>[6x]MGHHHHHHQQLASFLSGTWQSGRGRSRLIHHAISGEALWEVTSEGLDMAAARQFAIEKGAPALRAMTFIERAAMLKAVAKHLLSEKERFYALSAQTGATRADSWVDIEGGIGTLFTYASLGSRELPDDTLWPEDELIPLSKEGGFAARHLLTSKSGVAVHINAFNFPCWGMLEKLAPTWLGGMPAIIKPATATAQLTQAMVKSIVDSGLVPEGAISLICGSAGDLLDHLDSQDVVTFTGSAATGQMLRVQPNIVAKSIPFTMEADSLNCCVLGEDVTPDQPEFALFIREVVREMTTKAGQKCTAIRRIIVPQALVNAVSDALVARLQKVVVGDPAQEGVKMGALVNAEQRADVQEKVNILLAAGCEIRLGGQADLSAAGAFFPPTLLYCPQPDETPAVHATEAFGPVATLMPAQNQRHALQLACAGGGSLAGTLVTADPQIARQFIADAARTHGRIQILNEESAKESTGHGSPLPQLVHGGPGRAGGGEELGGLRAVKHYMQRTAVQGSPTMLAAISKQWVRGAKVEEDRIHPFRKYFEELQPGDSLLTPRRTMTEADIVNFACLSGDHFYAHMDKIAAAESIFGERVVHGYFVLSAAAGLFVDAGVGPVIANYGLESLRFIEPVKPGDTIQVRLTCKRKTLKKQRSAEEKPTGVVEWAVEVFNQHQTPVALYSILTLVARQHGDFVD

PaaZ is a fusion of N-terminal aldehyde dehydrogenase domain and C-terminal hydratase domain in a single polypeptide. The PaaZ structure containing six monomers can be described as a tri-lobed architecture.

The first of the PaaZ cryoEM maps did not have any bound ligand, which is defined here as the substrate-free structure. The map has an overall nominal resolution of 2.9 Å allowing the tracing of the complete polypeptide chain and assignment of residues after three-fold averaging. The model consists of residues 2-679 with the loop regions less well defined. The side chain density for some of the negatively charged residues are poor and the acidic residues were built using the best rotamer that does not create steric overlaps with the nearby residues. Several densities that could correspond to water or ions are observed but have not been modeled. The hydratase domain from three-dimers forms an inner core that holds the whole structure together, where each arm or module consists of a domain swapped dimer of PaaZ monomer and the dehydrogenase domain within the dimer is closer to the adjacent hydratase monomer. Three short helices (residues 449–459) from each monomer of the hydratase domain form two layers at this inner core. Another helix from each monomer lies perpendicular and wraps around these short helices, forming a tightknit unit. The distance between the active sites as measured from the side chains of C295 (active site of aldehyde dehydrogenase) and D561 (active site of hydratase), either from the same monomer or different monomers within a dimer, is symmetric and ~51 Å. In fact, 3D classification of cryoEM data of both substrate-free and ligand bound PaaZ reveals that more than 85% of the particles classify into one single class ruling out any large domain movement.>GGMEVLDLVTGPDSVTEIEAFLNPRMGQPPTPESLTEGGQYYGWSRGINLATSDTEDSPGNNTLPTWSMAKLQLPMLNEDLTCDTLQMWEAVSVKTEVVGSGSLLDVHGFNKPTDTVNTKGISTPVEGSQYHVFAVGGEPLDLQGLVTDARTKYKEEGVVTIKTITKKDMVNKDQVLNPISKAKLD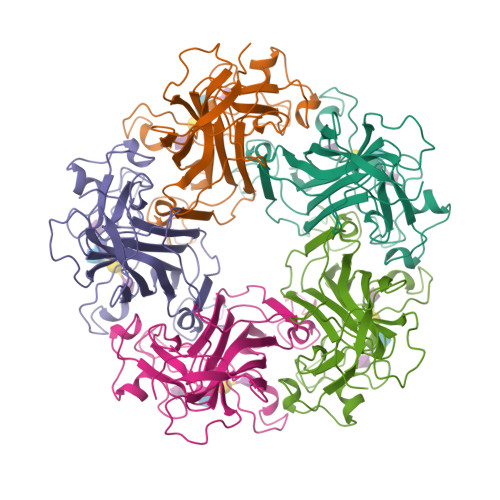KDGMYPVEIWHPDPAKNENTRYFGNYTGGTTTPPVLQFTNTLTTVLLDENGVGPLCKGEGLYLSCVDIMGWRVTRNYDVHHWRGLPRYFKITLRKRWVKNPYP[5x]>MAHHHHHHVDDDDKAASWSHPQFEKGAENLYFQSMLAAEAANRDHVTRCVAQTGGSPDLVAHTAALRLYLRVPHFLTEWTTDPDRRAAVSRALALDIVSMKLLDDLMDDDTGLDRVELACVCLRLHLRALHELESLARDPKAVTDILEQDAVHLCGGQIRTKRSRATNLREWRAHASTYGSTFLGRYGALAAACGGEGQ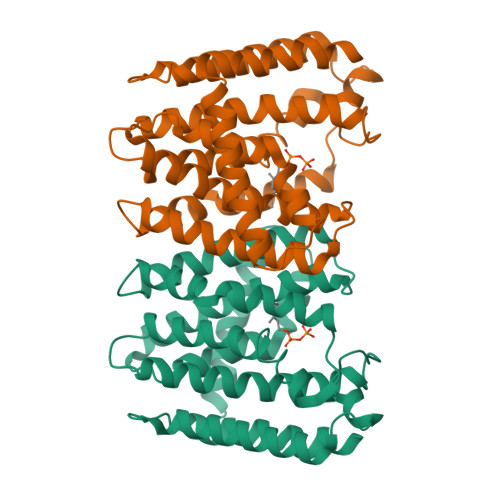PADSVREFAEAFAMTITMADDLTDYDRNGERDGNLAHLMRTGAVAGQDVVDLLEELRGRALAAVAAPPGAPGLVPVVHLYTDDVLVRLLPRHLGE[3x]> MSSGHHHHHHSYRVSTGAAHAAKGGGLVSGDSYSMMELGARKYAIAISDGMGNGARAHFESNETIKLLEKILESGIDEKIAIKTINSILSLRTTDEIYSTLDLSIIDLQDASCKFLKVGSTPSFIKRGDQVMKVQASNLPIGIINEFDVEVVSEQLKAGDLLIMMSDGIFEGPKHVENHDLWMKRKMKGLKTNDPQEIADLLMEEVIRTRSG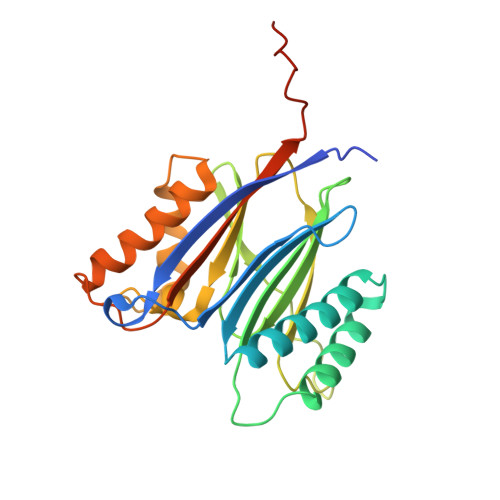QIEDDMTVVVVRIDHNTPKWASIPVPAIFQNKQEIS>[4x]MGSDK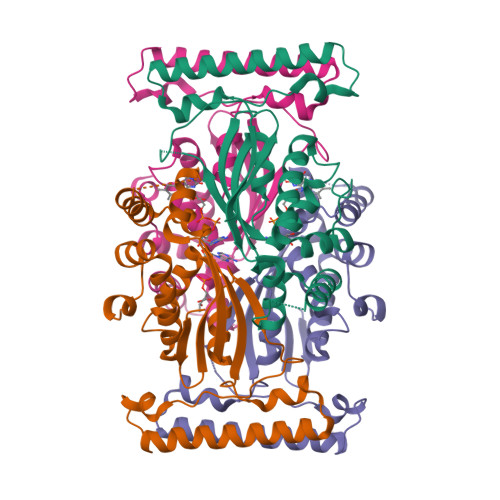IHHHHHHMKIDILDKGFVELVDVMGNDLSAVRAARVSFDMGLKDEERDRHLIEYLMKHGHETPFEHIVFTFHVKAPIFVARQWFRHRIASYNELSGRYSKLSYEFYIPSPERLEGYKTTIPPERVTEKISEIVDKAYRTYLELIESGVPREVARIVLPLNLYTRFFWTVNARSLMNFLNLKADSHAQWEIQQYALAIARIFKEKCPWTFEAFLKYAYKGDILKEVQV The long-wavelength beamline I23 at Diamond Light Source overcomes these limitations and extends the accessible wavelength range to λ = 5.9 Å. In this study, we report the determination of diverse protein structures by experimental phasing techniques carried out at long wavelengths on beamline I23 at Diamond Light Source using S, Ca, K, Cl, V, I, Cd, and P as anomalous scatterers. Native-SAD uses light atoms naturally occurring in proteins or bound to proteins. We demonstrate that long-wavelength native-SAD has become a very compelling technique, where a low multiplicity dataset from a single crystal can be sufficient for successful structure determination, making it a general vehicle of choice for experimental phasing.

The second method applies laser shaping of the crystal to remove all non-diffracting materials and define more regular path lengths through the crystals. Crystals of BphA4 complexed with FAD were shaped as spheres at SPring-8 (Japan) and collected at the phosphorus edge (λ = 5.76 Å) on beamline I23. At this wavelength, the anomalous signal from sulfur is negligible. Only the anomalous signal from the two phosphorus atoms of the FAD molecule was present to successfully phase BphA4, despite the low resolution of 3.7 Å (detector limited) and a low overall multiplicity of 12. Since the two phosphorus atoms are close to each other, they behave as a super-phosphorus with an anomalous peak height of 39.7 σ.

> MSQEALKAPVVVLGAGLASVSFVAELRQAGYQGLITVVGDEAERPYDRPPLSKDFMAHGDAEKIRLDCKRAPEVEWLLGVTAQSFDPQAHTVALSDGRTLPYGTLVLATGAAPRALPTLQGATMPVHTLRTLEDARRIQAGLRPQSRLLIVGGGVIGLELAATARTAGVHVSLVETQPRLMSRAAPATLADFVARYHAAQGVDLRFERSVTGSVDGVVLLDDGTRIAADMVVVGIGVLANDALARAAGLACDDGIFVDAYGRTTCPDVYALGDVTRQRNPLSGRFERIETWSNAQNQGIAVARHLVDPTAPGYAELPWYWSDQGALRIQVAGLASGDEEIVRGEVSLDAPKFTLIELQKGRIVGATCVNNARDFAPLRRLLAVGAKPDRAALADPATDLRKLAAAVAA>GSHMAGIGAAKVDTILEKDAYFPGEEVQGTVHVKGGKIAQDIRYIDLQLSTRYVIVKDDEEHRKYATIHSFRVTGSFTIQPGEEHQFPFTFTLPLDTPITVGKVEVAVVTDLDIQGGIDKSDHDRIFVEAHPWIENVLEAIENLGFRLNEADCEQAPYFQRRLPFVQEFEFVPTSGYYRQMLD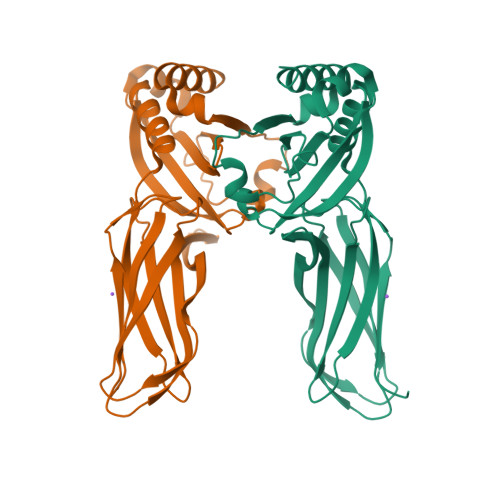ELELIFLLDEDGLEIIFEVDRRARGLRGWLEEMYNDGEQLVRVRFSQSELEDTEELEEVLEEILDQYAE[2x]> QRAKVAMSHFEPHEYIRYDLLEKNIDIVRKRLNRPL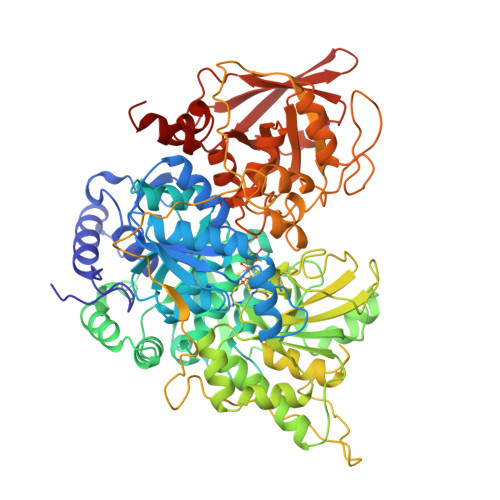TLSEKIVYGHLDDPANQEIERGKTYLRLRPDRVAMQDATAQMAMLQFISSGLPKVAVPSTIHCDHLIEAQLGGEKDLRRAKDINQEVYNFLATAGAKYGVGFWRPGSGIIHQIILENYAYPGVLLIGTDSHTPNGGGLGGICIGVGGADAVDVMAGIPWELKCPKVIGVKLTGSLSGWTSPKDVILKVAGILTVKGGTGAIVEYHGPGVDSISCTGMATICNMGAEIGATTSVFPYNHRMKKYLSKTGRADIANLADEFKDHLVPDPGCHYDQVIEINLSELKPHINGPFTPDLAHPVAEVGSVAEKEGWPLDIRVGLIGSCTNSSYEDMGRSAAVAKQALAHGLKCKSQFTITPGSEQIRATIERDGYAQVLRDVGGIVLANACGPCIGQWDRKDIKKGEKNTIVTSYNRNFTGRNDANPETHAFVTSPEIVTALAIAGTLKFNPETDFLTGKDGKKFKLEAPDADELPRAEFDPGQDTYQHPPKDSSGQRVDVSPTSQRLQLLEPFDKWDGKDLEDLQILIKVKGKCTTDHISAAGPWLKFRGHLDNISNNLLIGAINIENRKANSVRNAVTQEFGPVPDTARYYKQHGIRWVVIGDENYGEGSSREHSALEPRHLGGRAIITKSFARIHETNLKKQGLLPLTFADPADYNKIHPVDKLTIQGLKDFAPGKPLKCIIKHPNGTQETILLNHTFNETQIEWFRAGSALNRMKELQQK> MNLDTLLPLQTIREHAKCDDNPRV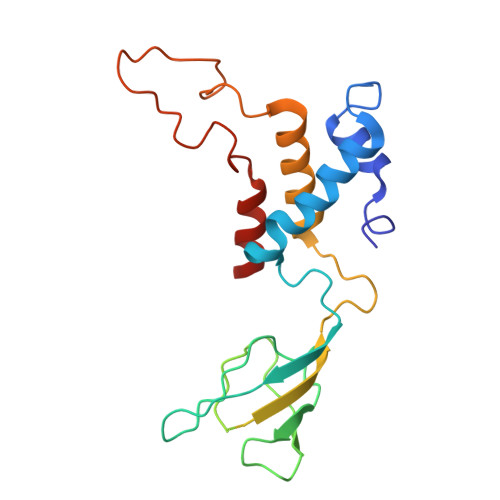TDDLLKLYREAAFEAAELYTGLSFTPEKTIVEPIRLKGRRGKIILSATPIAGRPVVFYGGGLGSPLELIPRPGSNVLFFPYGSPDRFQTWGDCHTCDVESQLMATYVTGRRCENSVPAGIIIGILKLIAWNINNPGDEVMSVRNTLNANAQGLIGGTNNGAVISGAQDEWFRYRRVLL> MGHHHHHHMVTQLKSASEYDSALASGDKLVVVDFF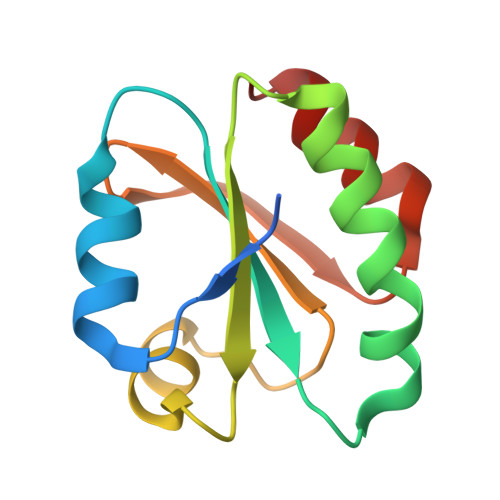ATWCGPSKMIAPMIEKFAEQYSDAAFYKLDVDEVSDVAQKAEVSSMPTLIFYKGGKEVTRVVGANPAAIKQAIASNV1-(1,2-benzoxazol-3-yl)methanesulfonamide 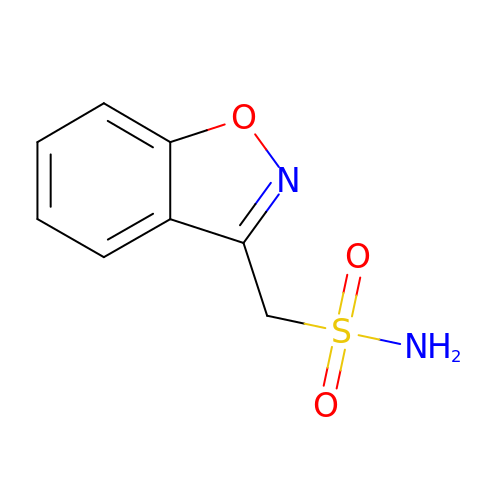| C8 H8 N2 O3 S | UBQNRHZMVUUOMG-UHFFFAOYSA-N> MKTEWPELVGKSVEEAKKVILQDK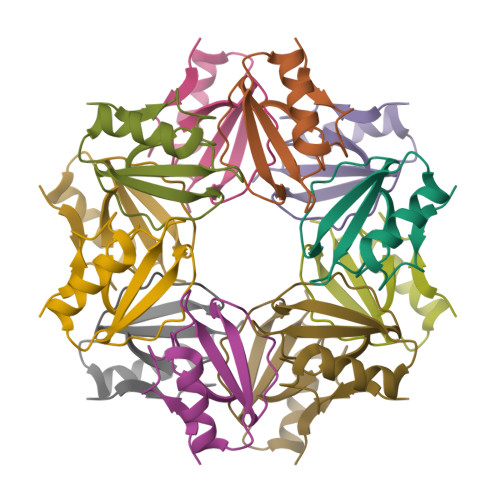PEAQIIVLPVGTIVTMEYRIDRVRLFVDKLDNVAEVPRVG>[4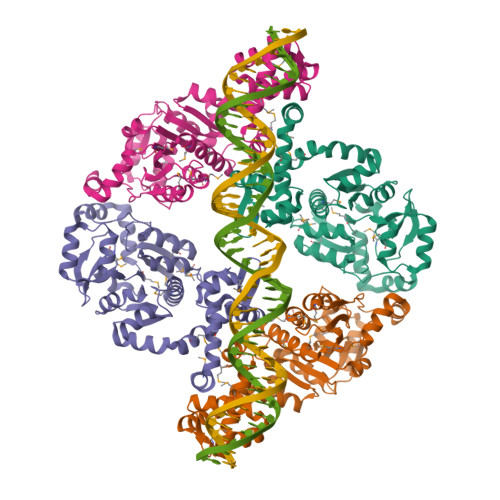x]GIDPFTMNQLIQAQKKLLPDLLLVMQKRFEILQYIRLTEPIGRRSLSASLGISERVLRGEVQFLKEQNLVDIKTNGMTLTEEGYELLSVLEDTMKDVLGLTLLEKTLKERLNLKDAIIVSGDSDQSPWVKKEMGRAAVACMKKRFSGKNIVAVTGGTTIEAVAEMMTPDSKNRELLFVPARGGLGEDVKNQANTICAHMAEKASGTYRLLFVPGQLSQGAYSSIIEEPSVKEVLNTIKSASMLVHGIGEAKTMAQRRNTPLEDLKKIDDNDAVTEAFGYYFNADGEVVHKVHSVGMQLDDIDAIPDIIAVAGGSSKAEAIEAYFKKPRNTVLVTDEGAAKKLLRDE> MRNKIFISHATPEDDDFTRWLSLKLIGLGYEVWCDILFLDKGVDFWSTIEKEIREN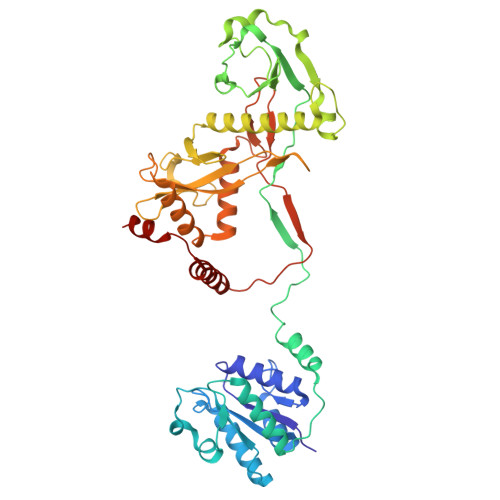TCKFLIVSSTAGNKREGVLKELAVATKVKKHLQDDMFIIPLAIDENLSYDDINIEIVRLNAIDFKKSWAKGLQDLLDAFEKQNVPKKPPDHSKSNLLYQQIFLHDKQAIEKEETYDSNWFPIISFPNELRFHRYDWRLPKQFDVRTLAFPAIRYKEYLCTFAWEYDFIHQLPKTETYNGQESIRISTSDILSGRYDTDFIRNYECQRLIVQLINKAFELRMKDKNVREYQMSKTFAYWIEKGKLEKDKFEKIKLVGKQKNKYWHFGISAAGKLYPSPVLMVSSHIIFTMDGINLIKSKSIQHSSRRKQGKNWWNDKWREKLLAFIRFLSDDQNAIYLNVGSEEKILISNKPLKFFGKMSYVTPSEVTLEEESVLADINNFEEDTEDLDELEDIE> MFDRYDAGEQAVLVHIYFTQDKDMEDLQEFESLVSSAGVEALQVITGSRKAPHPKYFVGEGKAVEIAEAVKATGASVVLFDHALSPAQERNLERLCECRVIDRTGLILDIFAQRARTHEGKLQVELAQLRHLATRLVRGWTHLERQKGGIGLRGPGETQLETDRRLLRNRIVQIQSRLERVEKQREQGRQSRIKADVPTVSLVGYTNAGKSTLFNRITEARVYAADQLFATLDPTLRRIDVADVGETVLADTVGFIRHLPHDLVAAFKATLQETRQATLLLHVIDAADVRVQENIEAVNTVLEEIDAHEIPTLLVMNKIDMLEDFEPRIDRDEENKPNRVW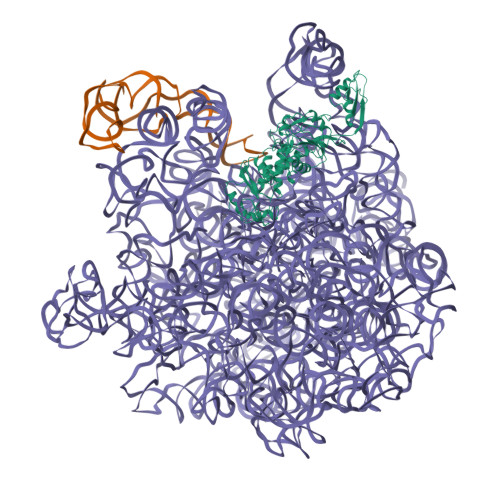LSAQTGAGIPQLFQALTERLSGEVAQHTLRLPPQEGRLRSRFYQLQAIEKEWMEEDGSVSLQVRMPIVDWRRLCKQEPALIDYLI Homologous recombination is a ubiquitous mechanism for maintaining genome integrity and also for generating genetic diversity in sexual reproductive organisms. This reaction is catalyzed by RecA family proteins, including bacterial RecA, archaeal RadA, and eukaryal Rad51 and Dmc1. The current model holds that, in the presence of ATP, the recombinases coat a primary single-stranded DNA (ssDNA) to form a nucleoprotein right-handed helical filament, and initiate a search for a secondary homologous stretches of double-stranded DNA (dsNDA). By contrast, archaeal RadA is a better model for eukaryotic recombinases.

Here we report additional three new crystal structures of left-handed helical filaments. First, the basic structural element of these three new helical filaments is a RadA dimer. The other protomers were then assigned as 2ZUB_B, 2ZUC_B and 2ZUD_B, respectively. A unique property of these left-handed helical filaments, as compared to other known structures of RecA family proteins, is that their DNA binding motifs (i.e., L1, L2 and NTD) are all located at the outermost surface of helical filaments. Moreover, the NTDs are separated a long way from L1 and L2 motifs. We found that the locations of the L1 and L2 motifs in the four left-handed helical filaments are relatively conserved, but in contrast, the NTD locations are quite different. The first hinge region, located between the NTD and the PM, is referred to here as “subunit rotational motif 1 (SRM1)”. Subsequent structural and biochemical analysis revealed that SRM1, a hinge region between the NTD and the PM, is not only responsible for structural flexibility of the NTD but also is important for RadA's function in promoting D-loop formation.

>MSNEVEQKKNIKTINDLPGISQTVINKLIEAGYSSLETLAVASPQDLSVAAGIPLSTAQKIIKEARDALDIRFKTALEVKKERMNVKKISTGSQALDGLLAGGIETRTMTEFFGEFGSGKTQLCHQLSVNVQLPPEKGGLSGKAVYIDTEGTFRWERIENMAKALGLDIDNVMNNIYYIRAINTDHQIAIVDDLQELVSKDPSIKLIVVDSVTSHFRAEYPGRENLAVRQQKLNKHLHQLTRLAEVYDIAVIITNQVMARPDMFYGDPTVAVGGHTLYHVPGIRIQLKKSRGNRRIARVVDAPHLPEGEVVFALTEEGIRDAEE[2x]>MAKILCVLYDDPITGYPKSYARADVPKIDHYPGGQTAPTPKQIDFTPGELLGSVSGELGLRKYLEGLGHTLVVTSDKEGEDSVFERELPDAEIVISQPFWPAYLTPERIAKAKKLKLAVTAGIGSDHVDLEAAIKNGITVAEVTYSNSISVSEHVVMMILSLVRNYIPSYQWVIKGGWNIADCVERSYDLEAMHVGTVAAGRIGLAVLKRLKPFDVKLHYFQRHRLPESVENELGLTYHPSVEDMVKVCDVVTINAPLHPGTLDLFNDELISKMKRGAYLVNTARGKICNRDAVVRALESGQLAGYAGDVWFPQPAPKDHPWRTMPHHGMTPHISGTSLSAQARYAAGTREILECWFEERPIREEYLIVDGGKLAGTGAHSYTVSK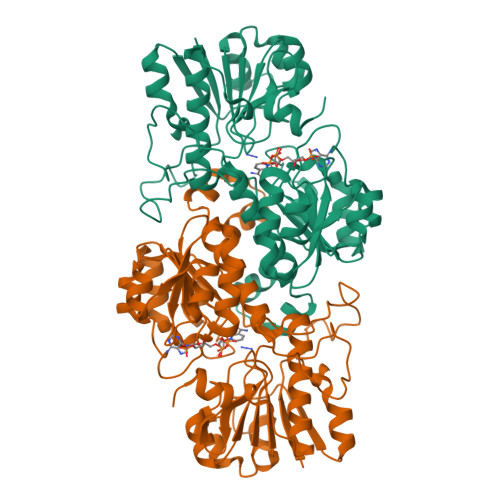[4x]> GHMERLLDELTLEGVARYMQSERCRRVICLVGAGISTSAGIPDFRSPSTGLYDNLEKYHLPYPEAIFEISYFKKHPEPFFALAKELYPGQFKPTICHYFMRLLKDKGLLLRCYTQNIDTLERIAGLEQEDLVEAHGTFYTSHCVSASCRHEYPLSWMKEKIFSEVTPKCEDCQSLVKPDIVFFGESLPARFFSCMQSDFLKVDLLLVMGTS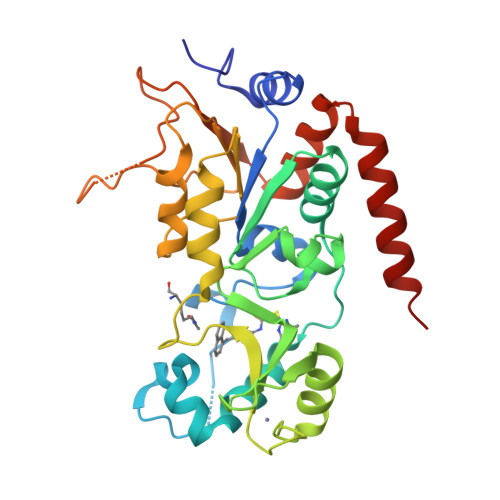LQVQPFASLISKAPLSTPRLLINKEKAGQSDPFLGMIMGLGGGMDFDSKKAYRDVAWLGECDQGCLALAELLGWKKELEDLVRREHASIDAQS;> TGGKAPR>[2x]HHMSELKIKAAKAAIAYIEDDMVIGVGTGSTVNFFIKELAAIKHKIEACVASSKATEALLRAEGIPVIDLN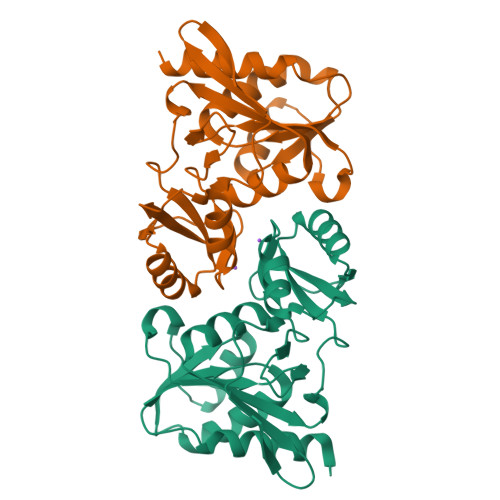SVQDLPIYVDGADEVNERGEMIKGGGGALTREKIVANVATQFICIVDESKVVKRLGEFPVAVEVIPMARSFVARQIVKLGGDPEYREGFVTDNGNIILDVFNLSFSTPMALEDSLNVIPGVVENGVFAKRLADKVLVASASGVNNLK> GSQSAGGAMNTQIVPDAATCPACLAEMNTPGERRYRYPFINCTHCGPRFTIIRAMPYDRPFTVMAAFPLCPACDKEYRDPLDRRFHAQPVACPECGPYLEWVSHGEHAEQEAALQAAIAQLKMGNIVAIKGIGGFHLACDARNSNAVATLRARKHRPAKP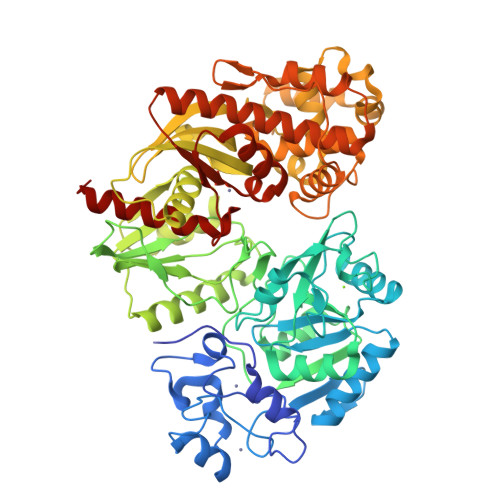LAVMLPVADGLPDAARQLLTTPAAPIVLVDKKYVPELCDDIAPGLNEVGVMLPANPLQHLLLQELQCPLVMTSGNLSGKPPAISNEQALEDLQGIADGFLIHNRDIVQRMDDSVVRESGEMLRRSRGYVPDALALPPGFKNVPPVLCLGADLKNTFCLVRGEQVVLSQHLGDLSDDGIQTQWREALRLMQNIYNFTPQYVVHDAHPGYVSCQWASEMNLPTQTVLHHHAHAAACLAEHQWPLDGGDVIALTLDGIGMGENGALWGGECLRVNYRECEHLGGLPAVALPGGDLAAKQPWRNLLAQCLRFVPEWQNYPETASVAAANWSVLARAIERGINAPLASSCGRLFDAVAAALGCAPATLSYEGEAACALEALAASCDGVTHPVTMPRVDNQLDLATFWQQWLNWQAPVNQRAWAFHDALAQGFAALMREQATMRGITTLVFSGGVIHNRLLRARLAHYLADFTLLFPQSLPAGDGGLSLGQGVIAAARWLAGE>[6x]MALAKRIDAALIVKDGRVVEGSNFENLRDSGDPVELGKFYSEIGIDELSFWDITASVEKRKTMLELVEKVAEQIDIPFTVGGGIHDFETASELILRGADKVEINTAA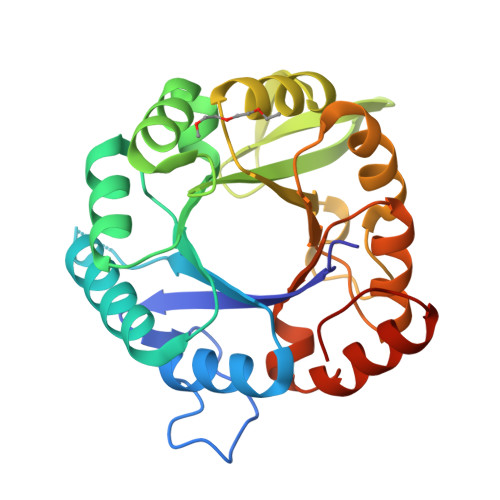VENPSLITQIAQTFGSQAVVVYIAAKRVDGEFMVFTYSGTKNTGILLRDWVVEVEKRGAGEIVLGSIDRLGTKSGYDTEMIRFVRPLTTLPIIAHRGAGKMEHFLEAFLAGADAAKADSVFHFREIDVRELKEYLKKHGVNVRLEGLGS> MDLTVEP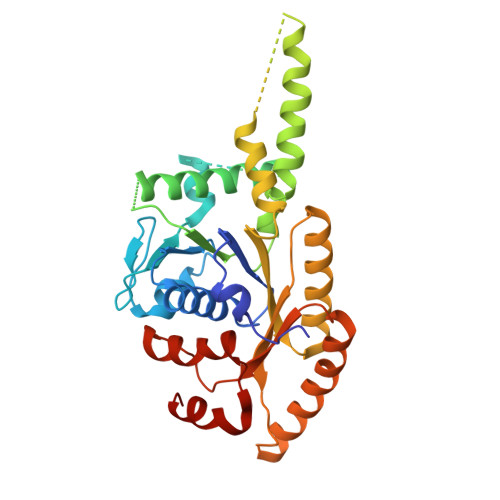NLHSLITSTTHKWIFVGGKGGVGKTTSSCSIAIQMALSQPNKQFLLISTDPAHNLSDAFGEKFGKDARKVTGMNNLSCMEIDPSAALKDMNDMAVSRANNNGSDGQGDDLGSLLQGGALADLTGSIPGIDEALSFMEVMKHIKRQEQGEGETFDTVIFDTAPTGHTLRFLQLPNTLSKLLEKFGEITNKLGPMLNSFMGAGNVDISGKLNELKANVETIRQQFTDPDLTTFVCVCISEFLSLYETERLIQELISYDMDVNSIIVNQLLFAENDQEHNCKRCQARWKMQKKYLDQIDELYEDFHVVKMPLCAGEIRGLNNLTKFSQFLNKEYNPITDGKVIYELEDKE>EELPQIEIVQEGDNTTFAKPGDTVTIHYDGKLTNGKEFDSSRKRGKPFTCTVGVGQVIKGWDISLTNNYGKGGANLPKISKGTKAILTIPPNLAYGPRGIPGIIGPNETLVFEVELLGVN[2x]

The 12-kDa FK506-binding protein (FKBP12) is a ubiquitously expressed peptidyl-prolyl isomerase with considerable homology between fungal pathogens and is thus a prime candidate for future targeting efforts to generate a panfungal strategy. PPIase proteins all catalyze the cis/trans isomerization of peptide bonds N terminal to proline residues in polypeptide chains. In addition to its role as a PPIase, FKBP12 is a member of the immunophilin family and is the target of the immunosuppressive drugs FK506 and rapamycin. Three extended loops, which have been called the 40s loop (between β2 and β3), the 50s loop (between β3′ and α1), and the 80s loop (between β4 and β5), surround a deep active-site pocket that binds both FK506 and rapamycin.

Interestingly, initial attempts to obtain crystals of the protein-FK506 complex failed, as the intermolecular interaction appeared to be strongly favored, leading to the production of the same apo crystal forms. Thus, we generated a P104G mutation in C. albicans FKBP12 and crystallized and obtained the apo FKBP12(P104G) structure to 2.0 Å. Strikingly, this structure did not harbor the self-catalysis-like interaction.> EPKQ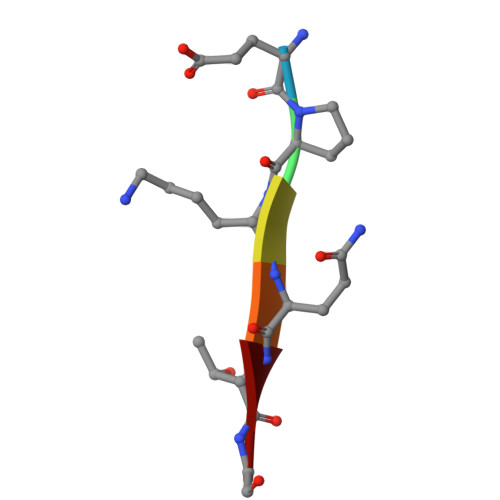TG> DEALAKAKGCMACHAIDKKLVGPSYKD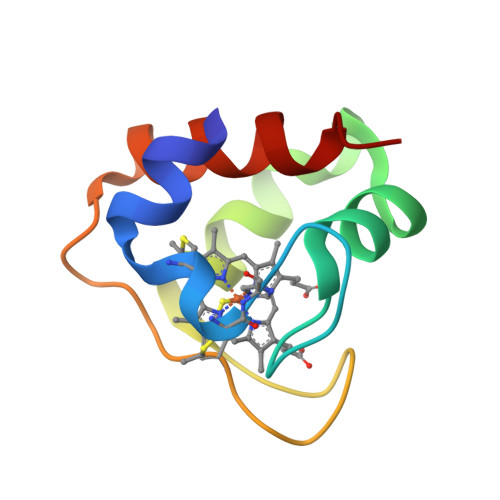VAKKYTEADVPKLVEKVKKGGAGVWGPVPMPPHPQVAEADIEKIVRWVLTLK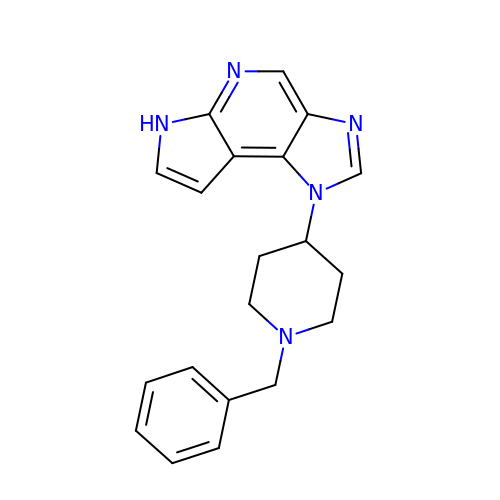1-(1-benzylpiperidin-4-yl)-1,6-dihydroimidazo[4,5-d]pyrrolo[2,3-b]pyridine | C20 H21 N5 | WKWXJWGOAKGEEM-UHFFFAOYSA-N>MIVFVRFNSSHGFPVEVDSDTSIFQLKEVVAKRQGVPADQLRVIFAGKELRNDWTVQNCDLDQQDIVHIVQRPWRKGQEMNATNSFYVYCKGPCQRVQPGKLRVQCSTCRQATLTLTQGPSCWDDVLIPNRMSGECQSPHCPGTSAEFFFKCGAHPTSDKETSVALHLIATNSRNITCITCTDVRSPVLVFQCNSRHVICLDCFHLYCVTRLNDRQFVHDPQLGYSLPCVAGCPNSLIKELHHFRILGEEQYNRYQQYGAEECVLQMGGVLCPRPGCGAGLLPEPDQRKVTCEGGNGLGCGFAFCRECKEAYHEGECSAV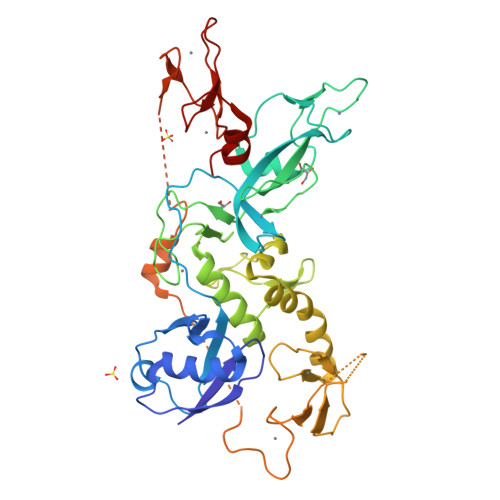FEASGTTTQAYRVDERAAEQARWEAASKETIKKTTKPCPRCHVPVEKNGGCMHMKCPQPQCRLEWCWNCGCEWNRVCMGDHWFDV[2x]>GHMSRRSFKNRVLAFFKGYPSFYYPATLVAPV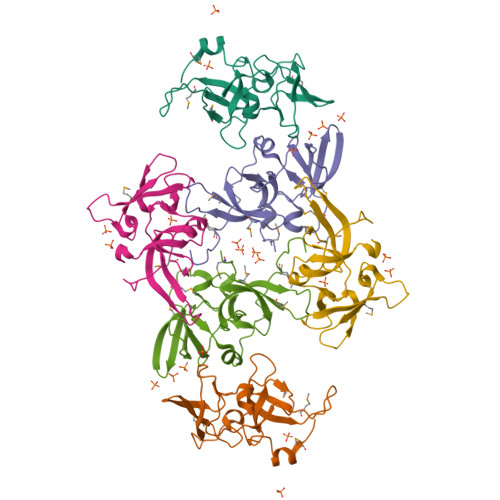HSAVTSSIMYKVQFDDATMSTVNSNQIKRFFLKKGDVVQSTRLGKIKHTVVKTFRSTNEQLSLIAVDALNNDMVILAHGEIEVTVPISTIYVAPVNIRRFQGRDLSFSTLKDMKFEETSFL[3x]> APTSSSTKKTQLQLEHLLLDLQMILNGINNYKNPKLT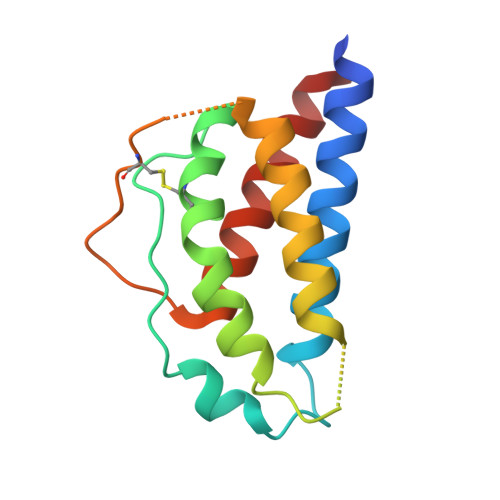RMLTFKFYMPKKATELKHLQCLEEELKPLEEVLNLAQSKNFHLRPRDLISNINVIVLELKGSETTFMCEYADETATIVEFLNRWITFCQSIISTLT>[2x]SSSSTASASAKKIIVKHVTVIGGGLMGAGIAQVAAATGHTVVLVDQTEDILAKSKKGIEESLRKVAKKKFAENPKAGDECVEKTLSTIATSTDAASVVHSTDLVVEAIVENLKVKNELFKRLDKFAAEHTIFASNTSSLQITSIANATTRQDRFAGLHFFNPVPVMKLVEVIKTPMTSQKTFESLVDFSKALGKHPVSCKDTPGFIVNRLLVPYLMEAIRLYERGDASKEDIDTAMKLGAG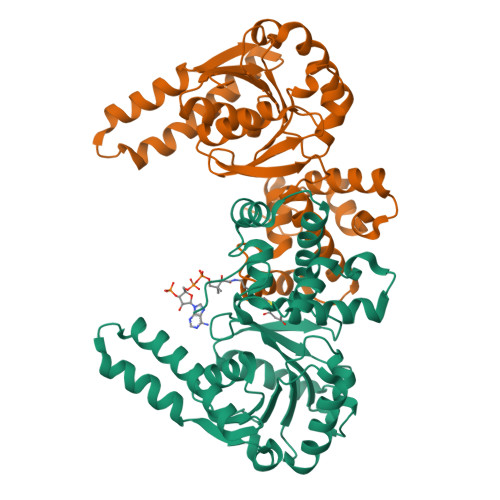YPMGPFELLDYVGLDTTKFIVDGWHEMDAENPLHQPSPSLNKLVAENKFGKKTGEGFYKYKLEHHHHHH>GAMDKAVGMSNDGRFLKFDIEIGRGSFKTVYKGLDTETTVEVAWCELQDRKLTKSERQRFKEEAEMLKGLQHPNIVRFYDSWESTVKGKKCIVLVTELMTSGTLKTYLKRFKVMKIKVLRSWCRQILKGLQFLHTRTPPIIHRDLKCDNIFITGPTGSVKIGDLGLATLKRASFAKSVIGTPEFMAPEMYEEKYDESVDVYAFGMCMLEMATSEYPYSECQNAAQIYRRVTSGVKPASFDKVAIPEVKEIIEGCIRQNKDERYSI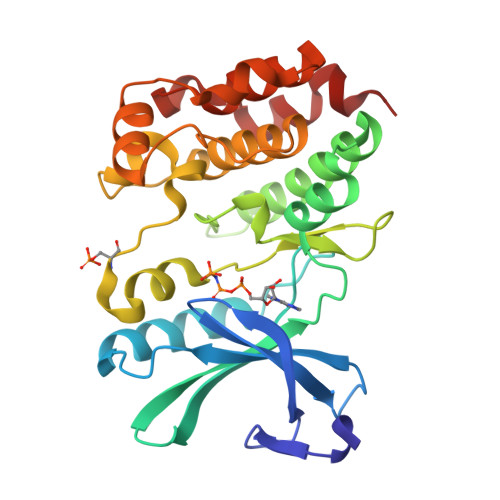KDLLNHAFFQEE[2x]>[2x]MAHHHHHHMQTLHVELGERR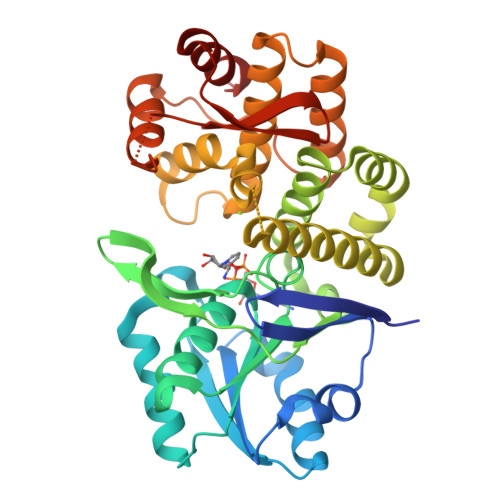YPIFIGSQLDPKQLLEPYIHGQQVMIVSNVTVAPLYLSHYQEALESLGKTVATCILPDGEKYKDIQHLNLIFDALLEAGFNRDCTVLALGGGVIGDMAGFASACFQRGVYFVQVPTTLLSQVDSSVGGKTGINHPLGKNMLGAFQQPQVVLADMAQLNTLPERELSAGLAEVIKYALLGDEDFLVWLEENMDGLVARDADLLAEAVYRSCAHKARIVANDEKEQGERALLNLGHTFGHAIESYLGYGTWLHGEAVATGMVMAADLSQRLGWISNEDVARTKKIIQRANLPISCPQIPLDDFLGYMAHDKKVLNGQLRLVLLKQLGQAVITKDFDVELMKQAILANQHG In the present study we report the discovery and the structural characterization of two novel flavoprotein oxidases from the thermophilic fungus M. thermophila. VAO-type proteins are composed of a FAD-binding domain and substrate domain. In both MtVAO615 and MtVAO713 the cofactor FAD is covalently tethered to the protein by covalent linkages.

The crystal structure of MtVAO615 with amino acid residues 27–574 was solved in two different space groups. The structure at pH 7.5 contains one monomer while the structure at pH 5.0 contains two monomers. Rcryst/Rfree are 19.5/23.5 and 23.6/28.0 respectively. As already observed by SDS-PAGE, MtVAO615 is heavily glycosylated, showing electron density in 2Fo-Fc maps for N-glycosylation at Asn47, Asn105, Asn129, Asn211, Asn310 and Asn438. As expected, MtVAO615 harbors a bicovalently linked 6-S-cysteinyl-8α-N1-histidyl FAD while MtVAO713 has a monocovalently linked 8α-methyl-N1-histidyl FAD. The isoalloxazine ring of the cofactor is covalently linked with the C6 atom to the Sγ of Cys222 and with the 8α-methyl group to the Nδ1 of His157 in MtVAO615 and His159 in MtVAO713. The groove shaped substrate binding pocket of MtVAO615 is solvent accessible and contains, besides His157 and Cys222 which tether the FAD, Tyr159, Thr221, His237, Thr341, Tyr352, Leu399, cis-Pro401, Ala402, cis-Pro403, Ala408, Phe410, Thr413, Tyr449, Asp451, Leu475 Ala477, Ala479, Glu519. On the other hand, despite having a bicovalently bound FAD cofactor, access to the active site of MtVAO615 is rather narrow. In particular, Phe410 and Tyr449 seem to create a sort of funnel. No other suitable reference dyes could be obtained. These observations indicate that the redox potential of MtVAO615 is extremely high for a flavoprotein, around 120–160 mV, which is close to the values reported for other bicovalent flavoproteins.

> MPASLLRFLALAGTAVGLTTNHNHSPSCRVLPGDAAWPSSRDWAKLNKTLNGHLIATVPQASVCHKSPFGQYDAQACEELKSSWDISTITHVNAPGDVLSQNFQNYSCVPFTDPSQPCQLGNYPSYVVNVTGAADVQAALKFAQKHNVRIVIKNTGHDYLGKSTGKGALSLWMHNLKSTKFIKNYKAPYYKGPAAKLGAGVEGFEAYAMANSTGHRIVGGTCPTVGIVGGYTQGGGHSILSSSYGVAADNVLEWEVVTADGRHLVATPTRNSDLYWALSGGGGGTFAVVLSMTARLHRDGIVGGTLLGFNDSAVGNEVYWEAVAAFHALLPDFLDGGNSFTYSVGNNSLTAYGTMPGADRDAVDRLLRPFLDDLASRGITPVVQPRVSTNYYDHFFTYLGPAPYGNAAYFPFTNSRIIPRSLVTDPKSNAVVTDLFRNISQVPAFSPFYCDSFSVADKPHPANSLHPAWRTGMLLCAPAGSWDWDASPEEMAARDRYAAETLQPMMDAATPGGSVYLNEANHLYANWKESFYGDNYARLLRVKKKYDPDSVFYVKTGVGSEVWDVDATGRLCRA> A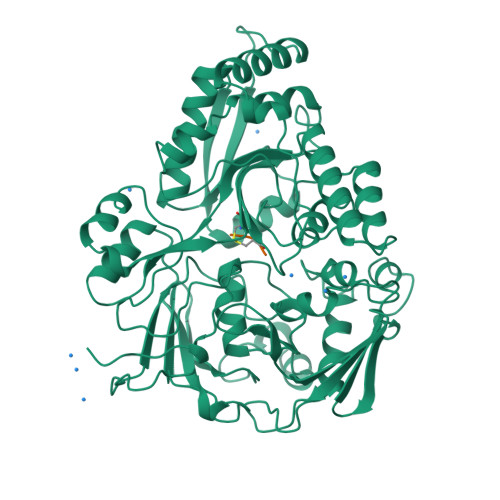DVPAGVQLADKQTLVRNNGSEVQSLDPHKIEGVPESNVSRDLFEGLLISDVEGHPSPGVAEKWENKDFKVWTFHLRENAKWSDGTPVTAHDFVYSWQRLADPNTASPYASYLQYGHIANIDDIIAGKKPATDLGVKALDDHTFEVTLSEPVPYFYKLLVHPSVSPVPKSAVEKFGDKWTQPANIVTNGAYKLKNWVVNERIVLERNPQYWDNAKTVINQVTYLPISSEVTDVNRYRSGEIDMTYNNMPIELFQKLKKEIPNEVRVDPYLCTYYYEINNQKAPFNDVRVRTALKLALDRDIIVNKVKNQGDLPAYSYTPPYTDGAKLVEPEWFKWSQQKRNEEAKKLLAEAGFTADKPLTFDLLYNTSDLHKKLAIAVASIWKKNLGVNVNLENQEWKTFLDTRHQGTFDVARAGWCADYNEPTSFLNTMLSDSSNNTAHYKSPAFDKLIADTLKVADDTQRSELYAKAEQQLDKDSAIVPVYYYVNARLVKPWVGGYTGKDPLDNIYVKNLYIIKH;> KFK> FKSTTQLIQQVSLTDFFRPDIEHAGSTVLILRHPTDLPALARHRAPPGRQTERLAEAWGQLLEASRAYVTSLSFIAACRAEEYTDKQAAEANRTAIVSAYGCSRMGARLIRFSECLRAMV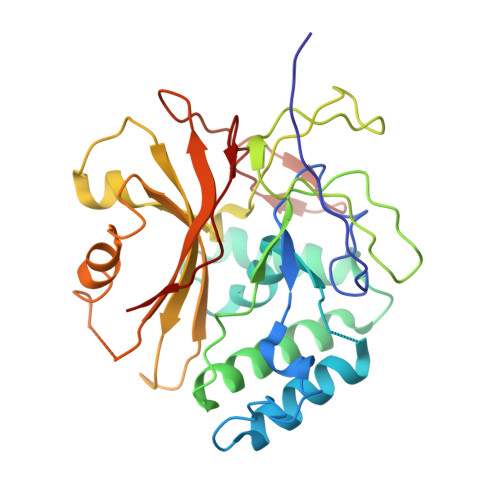QCHVFPHRFISFFGSLLEYTIQDNLCNITAVAKGPQEAARTDKTSTRRVTANIPACVFWDVDKDLHLSADGLKHVFLVFVYTQRRQREGVRLHLALSQLNEQCFGRGIGFLLGARICMYAAYTLIGTIPSESVRYTRRMERFGGYNVPTIWLEGVVWGGTNTWNEC> MPFVNKQFNYKDPVNGVDIAYIKIPNAGQMQPVKAFKIHNKIWVIPERDTFTNPEEGDLNPPPEAKQVPVSYYDSTYLSTDNEKDNYLKGVTKLFERIYSTDLGRMLLTSIVRGIPFWGGSTIDTELKVIDTNCINVIQPDGSYRSEELNLVIIGPSADIIQFECKSFGHEVLNLTRNGYGSTQYIRFSPDFTFGFEESLEVDTNPLLGAGKFATDPAVTLAHQLIHAGHRLYGIAINPNRVFKVNTNAYYEMSGLEVSFEELRTFGGHDAKFIDSLQENEFRLYYYNKFKDIASTLNKAKSIVGTTASLQYMKNVFKEKYLLSEDTSGKFSVDKLKFDKLYKMLTEIYTEDNFVKFFKVLNAKTFLNFDKAVFKINIVPKVNYTIYDGFNLRNTNLAANFNGQNTEINNMNFTKLKNFTGLFEFYKLLCVRGIITSKTKSLDKGYNKALNDLCIKVNNWDLFFSPSEDNFTNDLNKGEEITSDTNIEAAEENISLDLIQQYYLTFNFDNEPENISIENLSSDIIGQLELMPNIERFPNGKKYELDKYTMFHYLRAQEFEHGKSRIALTNSVNEALLNPSRVYTFFSSDYVKKVNKATEAAMFLGWVEQLVYDFTDETSEVSTTDKIADITIIIPYIGPALNIGNMLYKDDFVGALIFSGAVILLEFIPEIAIPVLGTFALVSYIANKVLTVQTIDNALSKRNEKWDEVYKYIVTNWLAKVNTQIDLIRKKMKEALENQAEATKAIINYQYNQYTEEEKNNINFNIDDLSSKLNESINKAMININKFLNQCSVSYLMNSMIPYGVKRLEDFDASLKDALLKYIYDNRGTLIGQVDRLKDKVNNTLSTDIPFQLSKYVDNQRLLSTFTEYIKNIINTSILNLRYESNHLIDLSRYASKINIGSKVNFDPIDKNQIQLFNLESSKIEVILKNAIVYNSMYENFSTSFWIRIPKYFNSISLNNEYTIINCMENNSGWKVSLNYGEIIWTLQDTQEIKQRVVFKYSQMINISDYINRWIFVTITNNRLNNSKIYINGRLIDQKPISNLGNIHASNNIMFKLDGCRDTHRYIWIKYFNLFDKELNEKEIK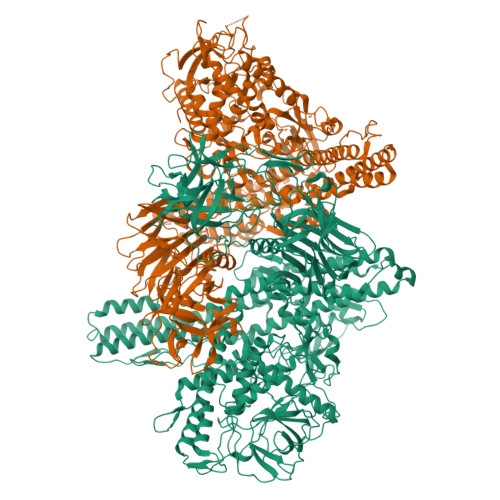DLYDNQSNSGILKDFWGDYLQYDKPYYMLNLYDPNKYVDVNNVGIRGYMYLKGPRGSVMTTNIYLNSSLYRGAKFIIKKYASGNKDNIVRNNDRVYINVVVKNKEYRLATNASQAGVEKILSALEIPDVGNLSQVVVMKSKNDQGITNKCKMNLQDNNGNDIGFIGFHQFNNIAKLVASNWYNRQIERSSRTLGCSWEFIPVDDGWGERPL;> GSMNINDNLSINSPVDNKNVVVVRARKTDTVFKAFKVAPNIWVAPERYYGESLSIDEEYKVDGGIYDSNFLSQDSEKDKFLQAIITLLKRINSTNAGEKLLSLISTAIPFPYGYIGGGYYAPNMITFGSAPKSNKKLNSLISSTIPFPYAGYRETNYLSSEDNKSFYASNIVIFGPGANIVENNTVFYKKEDAENGMGTMTEIWFQPFLTYKYDEFYIDPAIELIKCLIKSLYFLYGIKPSDDLVIPYRLRSELENIEYSQLNIVDLLVSGGIDPKFINTDPYWFTDNYFSNAKKVFEDHRNIYETEIEGNNAIGNDIKLRLKQKFRININDIWELNLNYFSKEFSIMMPDRFNNALKHFYRKQYYKIDYPENYSINGFVNGQINAQLSLSDRNQDIINKPEEIINLLNGNNVSLMRSNIYGDGLKSTVDDFYSNYKIPYNRAYEYHFNNSNDSSLDNVNIGVIDNIPEIIDVNPYKENCDKFSPVQKITSTREINTNIPWPINYLQAQNTNNEKFSLSSDFVEVVSSKDKSLVYSFLSNVMFYLDSIKDNSPIDTDKKYYLWLREIFRNYSFDITATQEINTNCGINKVVTWFGKALNILNTSDSFVEEFQNLGAISLINKKENLSMPIIESYEIPNDMLGLPLNDLNEKLFNIYSKNTAYFKKIYYNFLDQWWTQYYSQYFDLICMAKRSVLAQETLIKRIIQKKLSYLIGNSNISSDNLALMNLTTTNTLRDISNESQIAMNNVDSFLNNAAICVFESNIYPKFISFMEQCINNINIKTKEFIQKCTNINEDEKLQLINQNVFNSLDFEFLNIQNMKSLFSSETALLIKEETWPYELVLYAFKEPGNNVIGDASGKNTSIEYSKDIGLVYGINSDALYLNGSNQSISFSNDFFENGLTNSFSIYFWLRNLGKDTIKSKLIGSKEDNCGWEIYFQDTGLVFNMIDSNGNEKNIYLSDVSNNSWHYITISVDRLKEQLLIFIDDNLVANESIKEILNIYSSNIISLLSENNPSYIEGLTILNKPTTSQEVLSNYFEVLNNSYIRDSNEERLEYNKTYQLYNYVFSDKPICEVKQNNNIYLTINNTNNLNLQASKFKLLSINPNKQYVQKLDEVIISVLDNMEKYIDISEDNRLQLIDNKNNAKKMIISNDIFISNCLTLSYNGKYICLSMKDENHNWMICNNDMSKYLYLWSFKP1-[4-(5-chloropyrazin-2-yl)piperazin-1-yl]-2-[4-(propan-2-yl)phenyl]ethan-1-one | C19 H23 Cl N4 O | 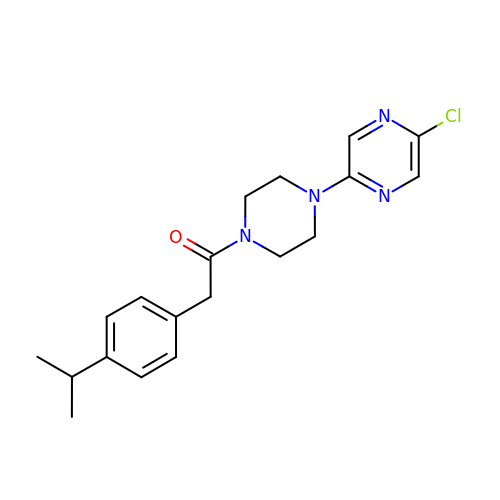ZABUHCOUTMKPGC-UHFFFAOYSA-N> MEKTEKNELVRKLIFNPQGDREASKRKIIKGNPTNIFELNEIKYSWAFDLYKLMGFTNFWIPEEIQMLEDRKQYETVLSDYEKRAYELVLSFLIALDSFQVDMLKEFGRMITAPEVEMAITAQEFQESVHAYSYQFILESVVDPVKADEIYNYWREDERLLERNKVIAELYNEFIRKPNEENFIKATIGNYILESLYFYSGFAFFYTLGRQGKMRNTVQQIKYINRDELCHVTLFRNIINTLRKENPELFTPEIEKWIVEYFKYAVNEEIKWGQYVTQNQILGINDVLIERYIKYLGNLRITQIGFDPIYPEVTENPLKWIDEFRKINNTKTDFFQAKPQTYSKANELKW

pmcThe enzyme ribonucleotide reductase (RNR) synthesizes the deoxyribonucleotides needed for DNA synthesis from their corresponding ribonucleotide precursors. Class I RNRs are composed of two proteins, a large α-subunit (R1) and a smaller β-subunit (R2) that exist as homodimers, that combine to form an active heterotetramer. Aquifex aeolicus is a hyperthermophilic bacterium with an unusual RNR encoding a 346-residue intein in the DNA sequence encoding its R2 subunit. We present the first structures of the A. aeolicus R1 and R2 (AaR1 and AaR2, respectively) proteins as well as the biophysical and biochemical characterization of active and inactive A. aeolicus RNR.

We expressed, purified, and determined the X-ray crystal structures of two AaR2 proteins: one in which the DNA sequence of the expressed protein lacked the intein (AaR2) and a second in which the nascent protein still included the intein sequence (AaR2_genomic). We crystallized the mature AaR2 and AaR2_genomic proteins and determined the X-ray crystal structures to resolutions of 1.73 and 2.10 Å, respectively. Superposition of AaR2 with AaR2_genomic shows the overall structures are virtually identical, with a low RMSD value of 0.15 Å. Analysis of the AaR2 di-iron site showed clear electron density for only one iron atom (termed Fe1), which was built in with an occupancy of 0.9. Fe1 is coordinated by three carboxylates (Glu127, Glu194, and Glu228), a histidine residue (His231), and one ordered water molecule. Interestingly, residues Glu127 and Glu194 display alternate conformations. Comparison of the AaR2 di-iron site with that of AaR2_genomic shows that the iron-coordinating residues occupy identical positions, with the exception of residues Glu194 and Glu127, which display alternate conformations in the AaR2 structure. However, it was evident that the presence of the intein in the construct seemed to influence the occupancy of the iron, particularly the Fe2 site, which had 25% occupancy in the AaR2_genomic structure but was empty in AaR2. The low tyrosyl radical content of AaR2 (0.05 Y•/AaR2) is likely the result of the low occupancy of iron in the active site.The second principal receptor for IgE, CD23, is a type II transmembrane glycoprotein with a C-type lectin-like domain (CTLD)4 (3, 4). In its membrane-bound form, CD23 consists of three CTLD “heads” connected to the membrane via a trimeric α-helical coiled-coil “stalk”. The interaction between CD23 and IgE is critical in the regulation of IgE synthesis, which can be up- or down-regulated depending on the oligomerization state of CD23 (2, 9, 10). We have determined the crystal structures of the human lectin-like head domain of CD23 in its Ca2+-free and Ca2+-bound forms, as well as the crystal structure of the Ca2+-bound head domain of CD23 in complex with a subfragment of IgE-Fc consisting of the dimer of Cϵ3 and Cϵ4 domains (Fcϵ3-4).

The S252A auxiliary binding site mutant crystallized in the same conditions and same crystal form as wild-type Ca2+-free derCD23. Similarly, Pro-250 is trans in two copies and cis in the others. As predicted from the crystal structure, the introduction of the S252A mutation did not affect Ca2+ binding, but unexpectedly, the D258A mutant was unable to bind Ca2+ even though the aspartate forms part of the apparently nonfunctioning auxiliary Ca2+-binding site. Ca2+ binding to the mutant derCD23 molecules (E249A and D270A, principal; S252A and D258A, auxiliary) was consistent with binding only to the principal site, with the exception of D258A, which showed no Ca2+ binding.

>SGFVCNTCPEKWINFQRKCYYFGKGTKQWVHARYACDDMEGQLVSIHSPEEQDFLTKHASHTGSWIGLRNLDLKGEFIWVDGSHVDYSNWAPGEPTARSQGEDCVMMRGSGRWNDAFCDRKLGAWVCDRLATCTPPASEGSAE[4x]> MAKHPVPKKKTSK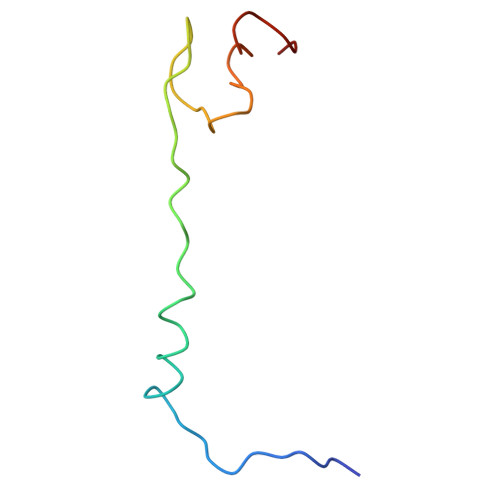SKRDMRRSHHALTAPNLTECPQCHGKKLSHHICPNCGYYDGRQVLAV> TPLGPASSLPQSFL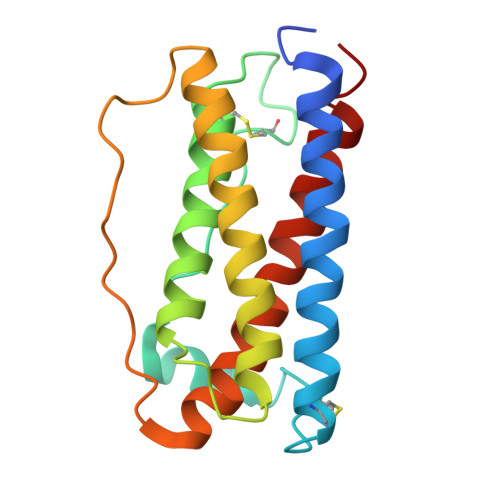LKCLEQVRKIQGDGAALQEKLCATYKLCHPEELVLLGHSLGIPWAPLSSCPSQALQLAGCLSQLHSGLFLYQGLLQALEGISPELGPTLDTLQLDVADFATTIWQQMEELGMAPALQPTQGAMPAFASAFQRRAGGVLVASHLQSFLEVSYRVLRHLAQP> ANNGLAITPQMGWNTWNKYGCNVDEQLILDAAKAIASSGLKDLGYNYVIIDDCWQKNERESSKTLLADPTKFPRGIKPLVDDIHNLGLKAGIYSSAGTLTCGGHIASLGYEDIDAKTWAKWGIDYLKYDNCYNQGQSGTPKLSYDRYKAMGNA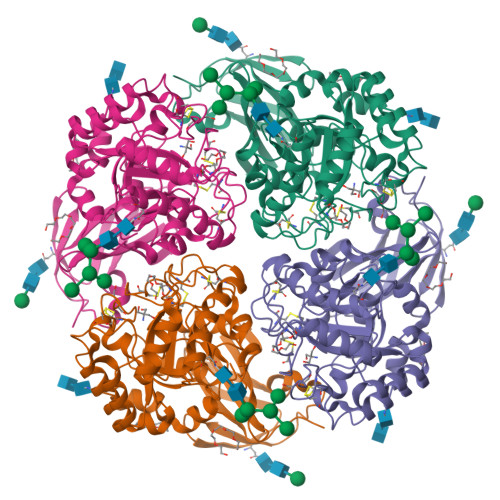LNKTGRPMLYSLCNWGEDGPWNFASTISNSWRISGDVYDNFNRPDPACPCTTYDCVLAGFRCSVMNIINKAVAVSQKARSGGWNDLDMLEVGNGGMNQEEYRVHYTIWAALKSPLILGNDVTNITNTTKEIIMNKEVIAVNQDSSFSPANRIWVKGDQQLFSGNLANNTQVVILLNAGDSAAKMTATWDDIWVYNLPNVDSSRSIEVRDLWKQKSLGNFSNHITLDVPAHGVRLLKFMDSATSS> GPGSNATQINEELYRLLEDTEILNQEITEGLLKGFEVPDAGVAIQLSKRDVVYPARILIIVLSEMWRFGLTKQSESFLAQVLTTIQKVVTQLKGNDLIPSGVFWLANVRELYSFVVFALNSILTEETF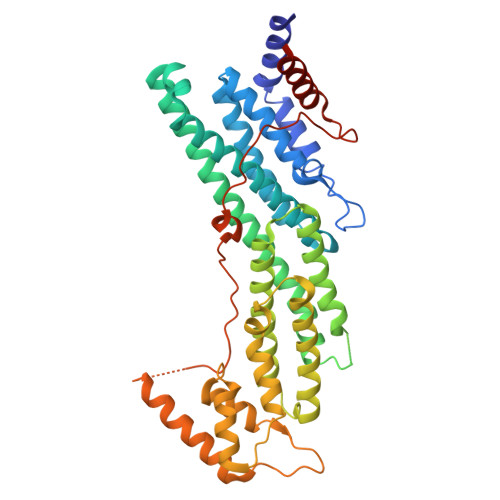KNGMTDEEYKEYVSLVTELKDDFEALSYNIYNIWLKKLQKQLQKKAINAVVISESLPGFSAGETSGANTEEYTMDDILTFFNSIYWCMKSFHIENEVFHAVVTTLLNYVDAICFNELIMKRNFLSWKRGLQLNYNVTRLEEWCKTHGLTDGTECLQHLIQTAKLLQVRKYTIEDIDILRGICYSLTPAQLQKLISQYQVADYESPIPQEILRYVADIVKKEAALSSSGNDSKGHEHSSSIFITPETGPFTDPFSLIKTRKFDQVEAYIPAWLSLPSTKRIVDLVAQQVVQDGHGSENLYFQ Rab proteins, the biggest subfamily within the superfamily of small GTPases, are major regulators of vesicular trafficking in eukaryotic cells. One such family of effector proteins that was reported to link Rab proteins and the cytoskeleton is the Mical (molecules interacting with CasL) family. In this publication, we present a thorough biochemical and structural analysis of a Rab effector domain termed bivalent Mical/EHBP Rab binding (bMERB) domain. The results show that the domains probably constitute a Rab8-effector family involved in endosomal trafficking, and the Rab-binding specificity can be well explained from the 3-dimensional structures of complexes determined in this work.

Well diffracting crystals were found using the RBD of Mical-cL (residues 534–683) in complex with different Rab proteins (Rab1, Rab8 and Rab10). In all structures (Rab1:Mical-cL, Rab8:Mical-cL and Rab10:Mical-cL) we found one Rab protein bound to one molecule of Mical-cL, in agreement with the previous observations that all Rab proteins tested bind only one site in Mical-cL. Most interactions were visible between the Rab proteins and α-helix 3 of Mical-cL with some additional contributing residues from α-helix 2, forming extensive contacts involving residues within switch I and II of the Rab proteins. In the Rab:Mical-cL structures, we observed extensive interaction of Mical-cL with RabSF1 (Tyr6, Asp7, Leu9, Lys11 in Rab10) and (less interactions) with RabSF2 (Asp31, Ser40 in Rab10). Accordingly, the sequence alignment of different Rab proteins shows strong conservation of the interacting amino acids within these motifs amongst Rab1 (Rab1a/b, Rab35) and Rab8 (Rab8a/b, Rab10, Rab13, Rab15) family members that interact with bMERB domains, but not for other Rab proteins (a comparative scheme of the residues involved in interactions in the different complexes is shown in Figure 5—figure supplement 1a). Interestingly, whereas Rab1 contains a glutamate near the N-terminus (Glu4), all Rab8 family members contain one or (in the case of Rab10) two lysine residues in this region that point towards a negatively charged patch in Mical-cL. In contrast to the main interacting helix α3, which adopts a similar position in all three structures, we observed slightly different orientations of the α-helices 1 and 2, adopting a position slightly further away from Rab1 compared to Rab8 and Rab10. (b) In all structures of Rab proteins in complex with Mical-cL, the N-termini of the Rab proteins point towards a negatively charged patch of Mical-cL (Rabs are shown in cartoon representation as above; the surface of Mical-cL is colored by charge, red – negative charge, blue – positive charge). The sequence of the N-terminal residues of each Rab protein is shown below the corresponding structure: Whereas Rab1 contains a negatively charged glutamate at position 4, Rab8 and Rab10 contain one or two lysine residues at position 3 or at position 3 and 4, respectively.

> GHMAKKTYDLLFKLLLIGDSGVGKTCVLFRFSDDAFNTTFISTIGIDFKIKTVELQGKKIKLQIWDTAGQERFHTITTSYYRGAMGIMLVYDITNGKSFENISKWLRNIDEHANEDVERMLLGNKCDMDDKRVVPKGKGEQIAREHGIRFFETSAKANINIEKAFLTLAEDILRKTPVKEPNSENVDISSGGGVTGWKSKCC;> GHMKQEELKRLYKAQAIQRQLEEVEERQRASEIQGVRLEKALRGEADSGTQDEAQLLQEWFKLVLEKNKLMRYESELLIMAQELELEDHQSRLEQKLREKMLKEESQKDEKDLNEEQEVFTELMQVIEQRDKLVDSLEEQRIREKAEDQHFES> RSRSKRLFVQLKSAAMTNFCYVTRKSPEKKNFRIALRKYDPGV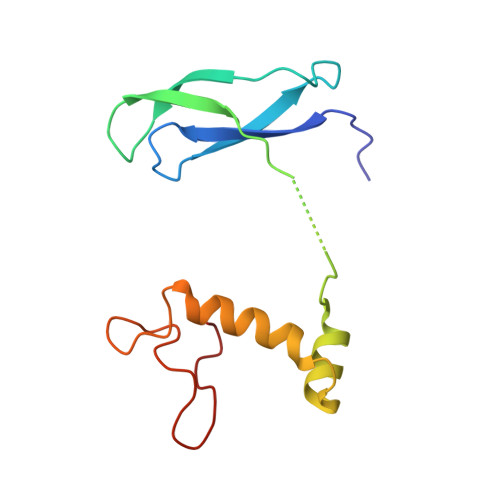NKHVMFYEARLPSEKNKKQITLSLQRYIRWTGKQVKLLLDKVEKAWEYGRFQKYFDNQAPLLTDRRGRAVPRYK> NVKEKSSEY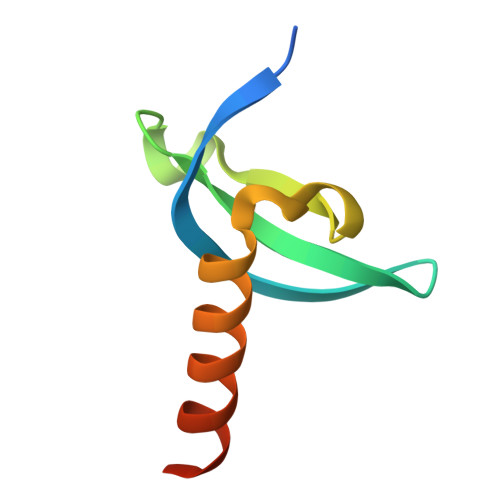IVEKFLGKRYLRGRPQYLTKWEGYPIEQCTWEPLENLGKCMTLIADYEAELFQQSREKKNDQ>[2x]MNKPQTIYEKLGGENAMKAAVPLFYKKVLADERVKHFFKNTDMD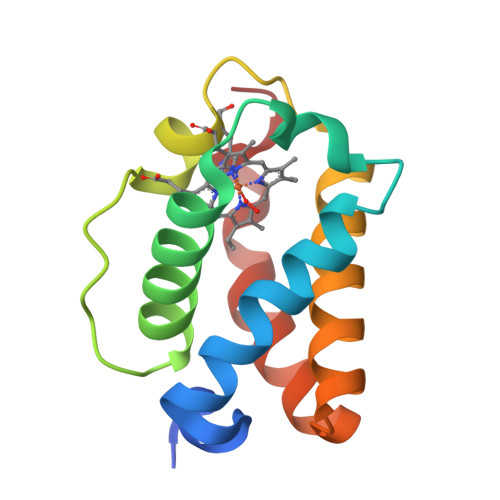HQTKQQTDFLTMLLGGPNHYKGKNMTEAHKGMNLQNLHFDAIIENLAATLKELGVTDAVINEAAKVIEHTRKDMLGK>[8x]AVPMLQDSVPLELDDAFMQDPHSVYARLNAEGSAHRVMMPPGVPVCGGLPVWLI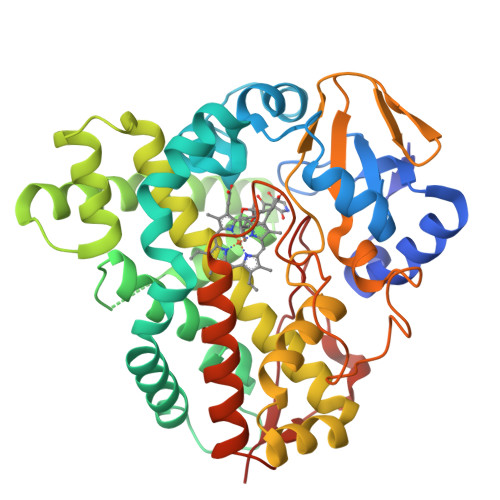TGYEEVRSALADPRLSTDLNRTDRLFAQNEPDRNKRGAFSSALATHMLHSDPPDHTRLRKLVNKAFTSRAIEKLRPEIEQITGELLAALPDEDPVDLLDAFAFPLPIRVICLLLGVPLEEQENFKSWSKALVSGDSPAATAAASTAMIEYLGDLIERKRRTPTDDVLAALVSARDVDDRLTETELVSMAFLLFIGGHETTVNTLGNGTLHLMRNLDQWEALRQDRSLLPGAVEEFLRLESPLKHATFRCATEDLRIGDTAIPAGDFVLLALASANRDPERFGDPHTLDVRRPTGGHVAFGHGIHYCLGAPLARMEAQVAFGVLLDTFPAMRLAVDPEDMRWRTSTLIRGLHSLPVRLNRP> GAGCAGACTTGACACCACTC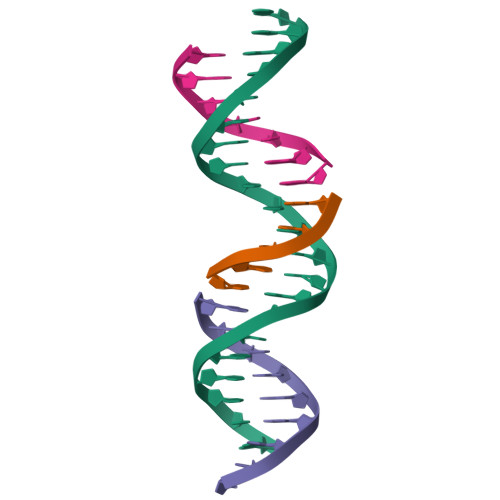A;> TGTCA;> TCTGAGTGA;> GGTCTGC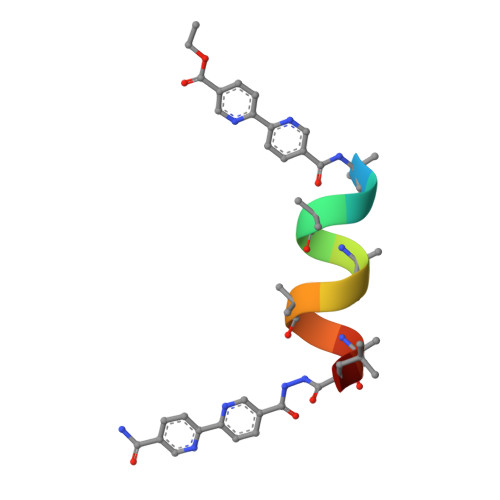>[2x]XALAAALAQALX> GSNNLNGMHLRLGIIPEMPFISEPSLGCTNIRDPSCYTGVNVEIVSMMSQDLNFTYNFITPEDLKFGGKNSTTGEWNGLIRDLLDNKTDMIVVALSNNAVRKADIDFSLSMMDGGLGALVKSDGTDLSHPLELLNQDKYQWG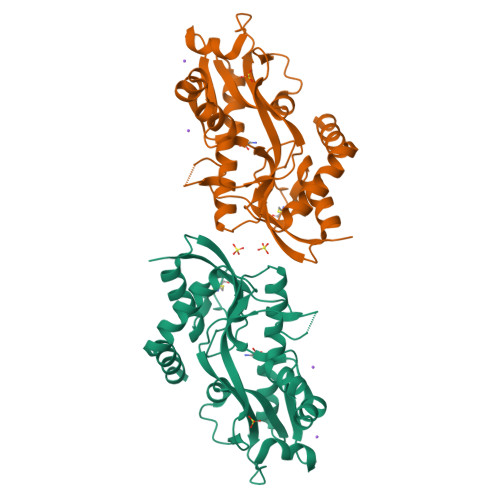VVDSRNPELLLASNQNADYNRIAEDAVKVGSYGEGLERMRAGGFVFIDEIPGINYATKGECDIVQIGETFQPFELAFGLRKNSPFKNLVDTFMLGIREQGVISELYAKYENQKASKPCN> SRKFIIANARVENCAVIYCNDGFCELCGYSRAEVMQ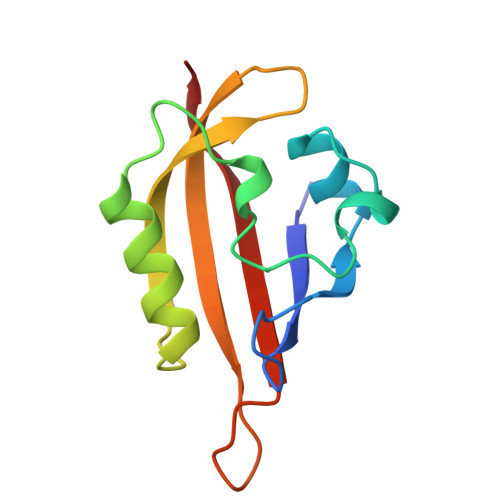RPCTCDFLHGPCTQRRAAAQIAQALLGAEERKVEIAFYRKDGSCFLCLVDVVPVKNEDGAVIMFILNFEVVMEK>MKAPVRVAVTGAAGQIGYSLLFRIAAGEMLGKDQPVILQLLEIPQAMKALEGVVMELEDCAFPLLAGLEATDDPKVAFKDADYALLVGAAPRKAGMERRDLLQVNGKIFTEQGRALAEVAKKDVKVLVVGNPANTNALIAYKNAPGLNPRNFTAMTRLDHNRAKAQLAKKTGTGVDRIRRMTVWGNHSSTMFPDLFHAEVDGRPALELVDMEWYEKVFIPTVAQRGAAIIQARGASSAASAA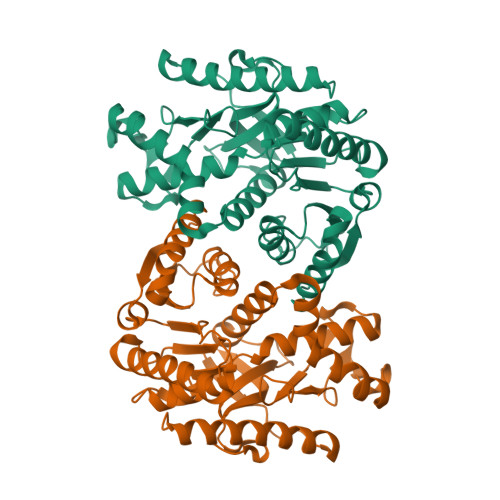NAAIEHIRDWALGTPEGDWVSMAVPSQGEYGIPEGIVYSFPVTAKDGAYRVVEGLEINEFARKRMEITAQELLDEMEQVKALGLI[2x]> MAMHLNENLDDNGEMHDINVTPFIDVMLVLLIIFMVAAPLA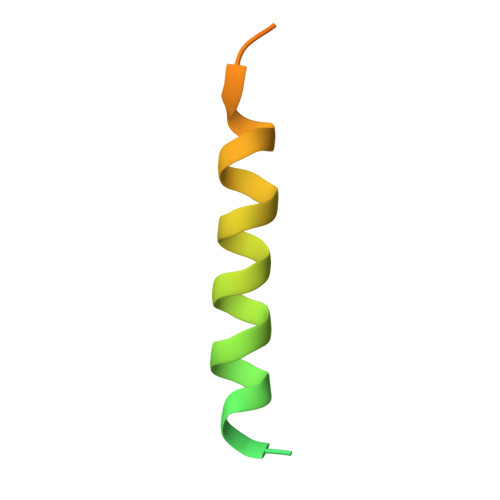TVDVKVNLGGGENLYFQ> MVLGTYKEIVSARSTDREIQKLAQDGGIVTGLLAYALDEGIIEGAVVAGPGEEFWKPQPMVAMSSDELKAAAGTKYTFSPNVMMLKKAVRQYGIEKLGTVAIPCQTMGIRKMQTYPFGVRFLADKIKLLVGIYCMENFPYTSLQTFICEKLGVSMELVEKM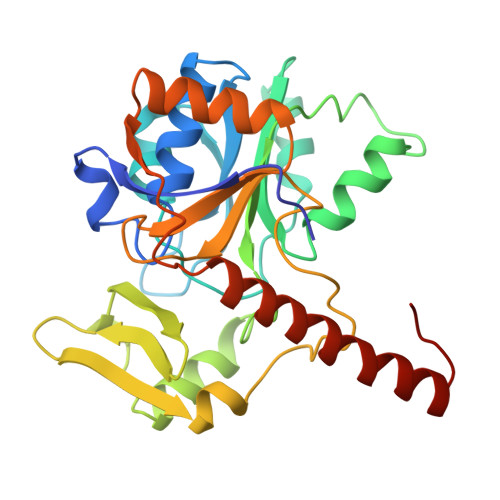DIGKGKFWVYTQDDVLTLPLKETHGYEQAGCKICKDYVAELADVSTGSVGSPDGWSTVITRTDAGDSIFKQAVEAGLFETKPIEEVKPGLGLLEKLAAQKKEKAEKNIAARKEMGLPTPF> GVATHGGSYVQYNVYGNLFEVSRKYVPPLRPIGRGAYGIVCAATNSETGEEVAIKKIGNAFDNIIDAKRTLREIKLLKHMDHENVIAVKDIIKPPQRENFNDVYIVYELMDTDLHQIIRSNQPLTDDHCRFFLYQLLRGLKYVHSANVLHRDLKPSNLLLNANCDLKLGDFGLARTKSETDFMTEYVVTRWYRAPELLLNCSEYTAAIDIWSVGCILGETMTREPLFPGKDYVHQLRLITELIGSPDDSSLGFLRSDNARRYVRQLPQYPRQNFAARFPNMSAGAVDLLEKMLVFDPSRRITVDEALCHPYLAPLHDINEEPVCVRP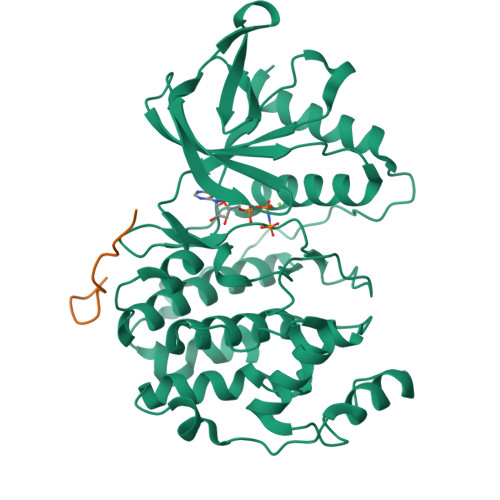FNFDFEQPTLTEENIKELIYRETVKFNP;> IHRDLKPSNLLIN>[8x]MAQPAAIIRIKNLRLRTFIGIK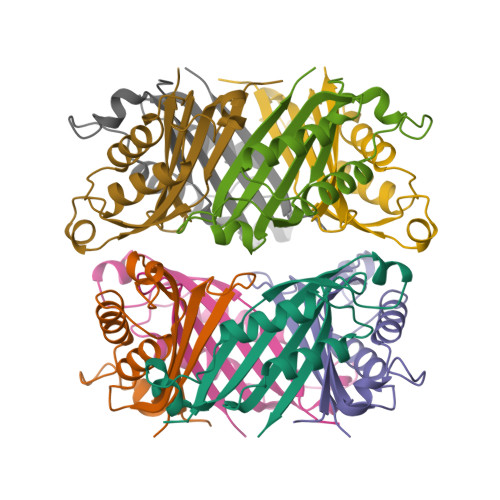EEEINNRQDIVINVTIHYPADKARTSEDINDALNYRTVTKNIIQHVENNRFSLLEKLTQDVLDIAREHHWVTYAEVEIDKLHALRYADSVSMTLSWQR N-({(2E)-2-[(4-chlorophenyl)methylidene]hydrazino}carbonothioyl)-beta-D-glucopyranosylamine | C14 H18 Cl N3 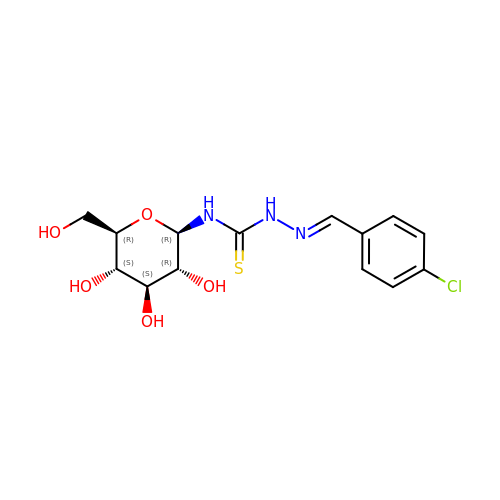O5 S | IRFPYSQRHIWLGT-QCOQDYPWSA-N>[2x]MSSEEKRLIKLPRTHKDGHLFEVSEAAIDWIEQYQHFKGVTKSIVELLNLISLRGLRSRDGLVSTTELIDATDGQLTRAAIQQRLRAAVAVGLFKQIPVRFEEGLAGKTMLHRFINPNQLIS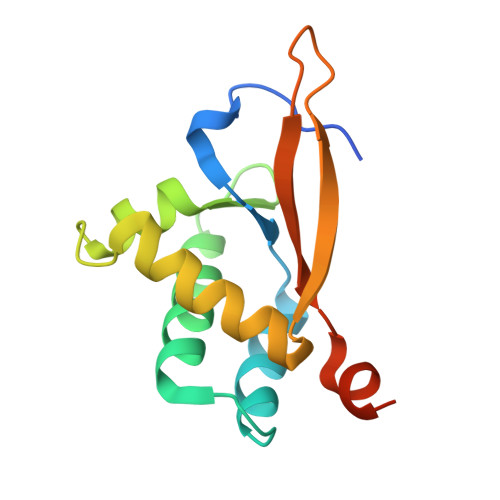VLHHHHHH>MSLPLLRPFETVSLENAVEDLVVRFILNVPPEDLSTVERVLFHFEEASWFYTDFVKLMNPYLPNLSIKSFSKIVIDICPLIWNWDITPENALVKFSNYKKTIPVRGAAIFNDSLSKILLLRGINSKHWSFPRGKIGKDEDDVACCIREVKEQTGFDLTGFIDADQYVERNMNGKNFKIFLVKGVPEDFEFKPEHKNEIQAIEWKDFKKLSKAITKNEGSAKVFLVNSMIRPLSLYVKNEKRAKDENKLKLYAEEHLKSILGLNKKENKIVLDAGR[2x];>GSMSTETLEIYRKALNFNVIARYDPKIKQLLFHTPHATVYKWGDDNWNKLEYQGVLAIYLRDVGDKEAILPEVSSYDDTITGQQSEANTPHVLTGHDIYNYGLIIMNRINPDNFSLAIAPNSVLNKRKLFAPNREEELEPMKVEVRDDLVMIKTLKKEVYGIWVHTPEDRQNIYELIKYLLENEPTDSFT[2x];>HSKCYAGATFATEAPQVTTLPKPSFV[2x];>MLNFKGYQIEIELKDGKRITGTLKQVSPKSLTLTDAVFQDGGVSPVFKIKADKLYDLKVLKLPPNA[2x]

Removal of the m7GpppN cap structure found at the 5′ end of all eukaryotic mRNA marks these transcripts for rapid clearance via the 5′-to-3′ mRNA decay pathway. The CD harbors a positively charged patch for RNA binding (box B motif)25,26 and a Nudix motif with conserved Glu residues that bind magnesium and carry out cap hydrolysis chemistry. The NRD enhances decapping activity by specifically recognizing the m7G nucleotide of cap and binding Dcp1, which further accelerates decapping. The activity of the core Dcp1–Dcp2 complex can be further modulated by the enhancer of decapping proteins (Edcs).

In this study, we present a new, four-protein structure of K. lactis Edc1–Dcp1–Dcp2–Edc3 at 2.84 Å resolution in the catalytically active conformation with bound substrate analog poised for catalysis. To trap the substrate-bound active conformation, we screened different Dcp1–Dcp2 constructs (S. pombe, K. lactis, H. sapiens) in which the catalytic Glu was mutated to Gln to prevent cap hydrolysis for co-crystallization with magnesium, a tight-binding two-headed cap analog, and coactivators Edc1 and Edc3. Edc3 Lsm domain binds an extended helix at the C-terminus of the Dcp2 CD, as in the recent Kl Dcp1–Dcp2–Edc3 structure, and the fully ordered Edc1 activation peptide bridges Dcp1 and Dcp2, similar to the recent Sp Edc1–Dcp1–Dcp2 structure. The conserved YAGxxF Dcp2-activating motif creates a 3-way interface that bridges Dcp1, Dcp2 NRD, and Dcp2 CD in the catalytically active conformation by threading through a narrow channel between these domains. Tyr359 of Kl Edc1, the residue most critical for activation, makes a cation–π interaction with the strictly conserved Arg39 on the Dcp2 NRD. Ala360 packs against conserved hydrophobic residues in the flexible hinge between Dcp2 NRD and CD, and Phe364 plugs into a pocket at the Dcp1–Dcp2 NRD interface consisting of positively charged and hydrophobic residues. Two-headed cap substrate analog bound at the Dcp2 active site engages conserved residues on the Dcp2 NRD and CD. In the active conformation reported here however, the CD is rotated ~90° from the pre-catalytic conformation, and Phe223 base stacks with the second m7G of our two-headed substrate analog, likely mimicking binding of the first transcribed nucleotide of RNA substrate to the Dcp2 CD. In the substrate analog-bound state, the β-phosphate, which undergoes nucleophilic attack by water during cap cleavage, is located 5.4 Å from the general base Glu152. In our substrate analog-bound structure, we were able to build one magnesium atom that is coordinated by Glu148.>MHIPADSFSGAS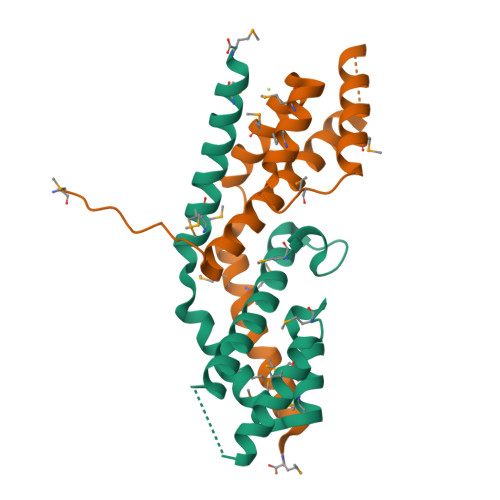PERKAAVALRSLFTFVAARVVLEQLQGPGGPETTYNQQAYLDLMDFLGTPMKGDGGDEWMAAVMRKNHALALRLMEVREAYLDEFEWGKTMEMASRETREANTRLMRAAAM[4x]>MATQGVFTLPANTRFGVTAFANSSNTQTVNVLVNNETAATFSGQSTNNAVIGTQVLNSGSSGKVQVQVSVNGRPSDLVSAQVILTNELNFALVGSEDGTDNDYNDAVVVINWPLG[4x]

The present study is devoted to the PA-IIL lectin from Pseudomonas aeruginosa, an opportunistic human pathogen capable of causing lethal complications in cystic fibrosis patients. The lectin may play an important role in the process of virulence, recognizing specific saccharide structures and subsequently allowing the bacteria to adhere to the host cells. It displays high values of affinity towards monosaccharides, especially fucose – a feature caused by unusual binding mode, where two calcium ions participate in the interaction with saccharide. Briefly, the structure is tetrameric with each monomer characterized by a binding site containing two calcium ions and a saccharide.

Hence, amongst the four monomers that form the asymmetric unit, substitution of the sugar occurred in the four monomers of PA-IIL S23A/Me-α-Fuc and G24N/Me-α-Man, but only in three monomers of the S22A/Me-α-Man and S22A/Me-α-Fuc complexes and in only two monomers of G24N/Me-α-Fuc. The other two monomers of G24N/Me-α-Fuc are lacking both calcium ions and don't contain any sugar moiety in the binding site. In the case of the G24N mutation, no new interaction is observed. The mutants S23A and G24N show approximately 200% and 160% higher affinity compared to PA-IIL, whose dissociation constant equals 430 nM. As for the mutant G24N, the situation is slightly different. There are no apparent new interactions observed and the two fold increase in affinity is therefore difficult to rationalize. While enthalpic contribution is almost the same, the entropy term becomes less unfavourable (difference of about 3 kJ/mol), which could imply that the mutant protein shows better surface complementarity to the interacting sugar. The side chain of Asp 24 makes an additional hydrogen bond with carboxylic group of Asp96 and closes the binding pocket that therefore cannot accommodate any further water molecule that is seen in all four binding sites of the wild type protein in proximity of Asp96.>MFVALGAQIYRQYFGRRGMAMANNSSVANKVCLIVIDGWGVSEDPYGNAILNAQTPVMDKLCSGNWAQIEAHGLHVGLPEGLMGNSEVGHLNIGAGRVIYQDIVRINLAVKNNKFVTNESLVDACDRAKNGNGRLHLAGLVSDGGVHSHIDHMFALVKAIKELGVPELYLHFYGDGRDTSPNSGVGFLEQTLEFLEKTTGYGKLATVVGRYYAMDRDNRWERINVAYEAMIGGVGETSDEAGVVEVVRKRYAADETDEFLKPIILQGEKGRVQNDDTIIFFDYRADRMREISAAMGMDRYKDCNSKLAHPSNLQVYGMTQYKAEFPFKSLFPPASNKNVLAEWLAEQKVSQFHCAETEKYAHVTFFFNGGLEKQFEGEERCLVPSPKVATYDLQPEMSAAGVADKMIEQLEAGTHPFIMCNFAPPDMVGHTGVYEAAVKACEATDIAIGRIYEATQKHGYSLMVTADHGNAEKMKAPDGGKHTAHTCYRVPLTLSHPGFKFVDPADRHPALCDVAPTVLAIMGLPQPAEMT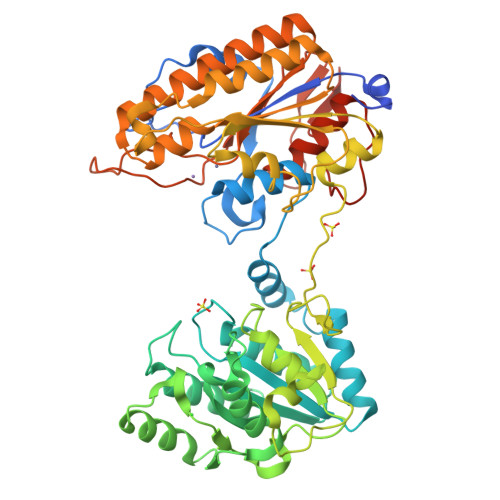GVSIVQKIKLAAALEHHHHHH[2x]>VLIAIEGVDGAGKRTLVEKLSGAFRAAGRSVATLAFPRYGQSVAADIAAEALHGEHGDLASSVYAMATLFALDRAGAVHTIQGLCRGYDVVILDRYVASNAAYSAARLHENAAGKAAAWVQRIEFARLGLPKPDWQVLLAVSAELAGERSRGRAQRDPGRARDNYERDAELQQRTGAVYAELAAQGWGGRWLVVGADVDPGRLAATLAPPDVPS[2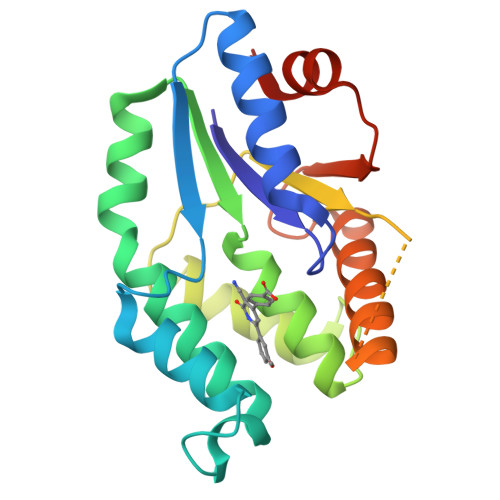x]>[2x]MNTTPVHALTDIDGGIAVDPAPRLAGPPVFGGPGNDAFDLAPVRSTGREMLRFDFPGVSIGAAHYEEGPTGATVIHIPAGARTAVDARGGAVGLSGGYDFNHAICLAGGAGYGLEAGAGVSGALLERLEYRTGFAELQLVSSAVIYDFSARSTAVYPDKALGRAALEFAVPGEFPQGRAGAGMSASAGKVDWDRTEITGQGAAFRRLGDVRILAVVVPNPVGVIVDRAGTVVRGNYDAQTGVRRHPVFDYQEAFAEQVPPVTEAGNTTISAIVTNVRMSPVELNQFAKQVHSSMHRGIQPFHTDMDGDTLFAVTTDEIDLPTTPGSSRGRLSVNATALGAIASEVMWDAVLEAGK

Nylon hydrolase (NylC) is one of the three enzymes responsible for the endo-type degradation of the by-products of nylon-6 manufacture (cyclic and linear oligomers of 6-aminohexanoate (Ahx) with a degree of polymerization greater than three) and various aliphatic nylons (e.g., nylon-6 and nylon-66). However, the post-translational autocleavage of the nascent polypeptide between Asn266 and Thr267 generates an active enzyme with an α subunit (27 kDa) and a β subunit (9 kDa). Based on the X-ray-crystallographic structure of NylCA, we reported that four αβ heterodimers (molecules A-D) form a doughnut-shaped quaternary structure. In addition, we proposed that the nucleophilic N-terminal residue Thr267 in the β subunit functions as a catalytic residue for either autocleavage (from precursor to active enzyme) or substrate hydrolysis.

His130 and Leu137 in NylCp2 were located in a loop between helix α1 and β-strand β7 (designated “loop 3”). Moreover, the temperature factors (index of thermal motion in a crystallographic structure) of loop regions 1–3 in NylCp2 were significantly larger than those of the corresponding regions in the thermostable NylC-G122Y130 mutant. In the thermostable enzymes, loop 3 and η3 (in monomer A) was mutually stabilized by contacts with loop 1 and loop 4 in monomer D. We found that the V225M substitution, which was close to Gln299, decreased the expression and/or stability of NylCp2 in cells, whereas this mutation increased the stability of NylC-G122Y130 by 2 °C9.> STYTQTKYPIVLAHGMLGFDNILGVDYWFGIPSALRRDGAQVYVTEVSQLDTSEVRGEQLLQQVEEIVALSGQPKVNLIGHSHGGPTIRYVAAVRPDLIASATSVGAPHKGSDTADFLRQIPPGSAGEAVLSGLVNSLGALISFLSSGSTG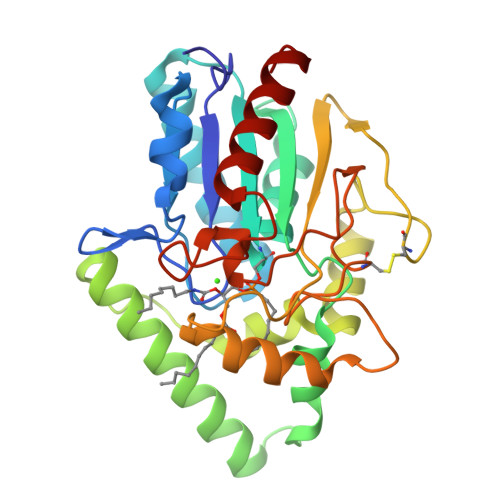TQNSLGSLESLNSEGAARFNAKYPQGIPTSACGEGAYKVNGVSYYSWSGSSPLTNFLDPSDAFLGASSLTFKNGTANDGLVGTCSSHLGMVIRDNYRMNHLDEVNQVFGLTSLFETSPVSVYRQHANRLKNASL>ESYCGPCPKNWICYKNNCYQFFDESKNWYESQASCMSQNASLLKVYSKEDQDLLKLVKSYHWMGLVHIPTNGSWQWEDGSILSPNLLTIIEMQKGDCALYASSFKGYIENCSTPNTYICMQRTV[2x];> DAHSLWYNFT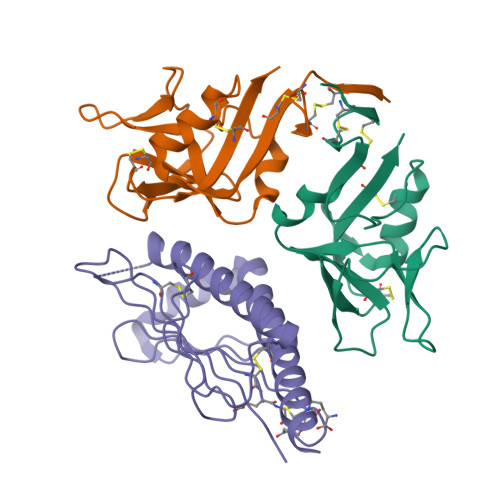IIHLPRHGQQWCEVQSQVDQKNFLSYDCGSDKVLSMGHLEEQLYATDAWGKQLEMLREVGQRLRLELADTELEDFTPSGPLTLQVRMSCEXEADGYIRGSWQFSFDGRKFLLFDSNNRKWTVVHAGARRMKEKWEKDSGLTTFFKMVSMRDCKSWLRDFLMHRKKRLE>STLPTPDDLMRRFIVKDTLITIFRRHGAVEAPTATLYPKSSHYGPNAVHLLDRNGTVLQLP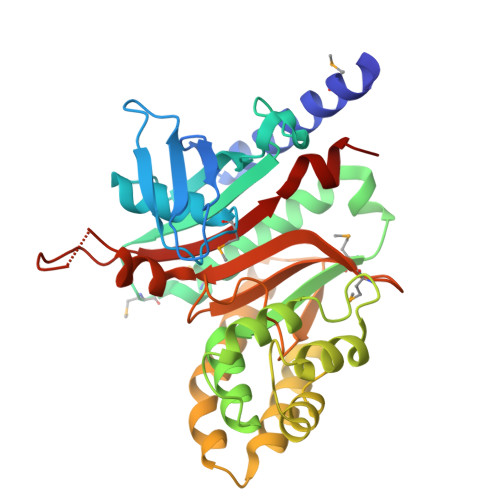FDLVMGHARSLARIASGPVPQRAYSFGNIFRDRQDGGQPDVYGEVDFDIVTTDAMDLAMKEAEVIKVLDEIIAAFPTTSSTPMCFQLGHSDLLQLIFDFCNVEHGARQAAAEVLSKLNIRNFTWQKVRSELRSPLVGISATSVDELQRFDWRDTPTKAFTKIRNLFEGTEYYDKVSSTLAHLKEVYEYSKKFKVNTKIYIAPLSSINEAFFRGGILFSCLYDRKVMDVFAAGGRYDGLIKAHRPRIGSRFEERHAVGFSLNWEKQLAKP[4x]>SNVRATYTVIFKNASGLPNGY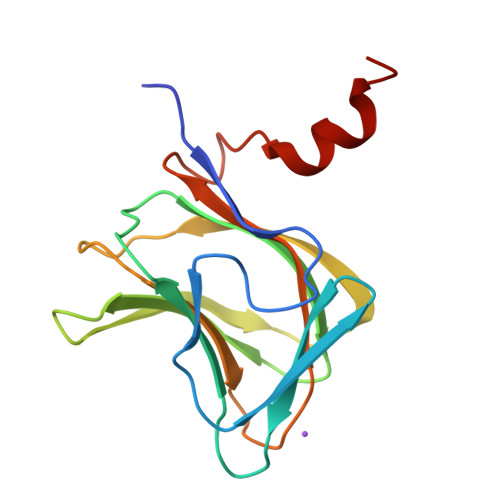DNWGWGCTLSYYGGAMIINPQEGKYGAVSLKRNSGSFRGGSLRFDMKNEGKVKILVENSEADEKFEVETISPSDEYVTYILDVDFDLPFDRIAFQDAPGNGDRIWIKNLVHSTGSADDFVDPINLEHHHHHH[2x]>EARPKIGLVLSGGAARGLAHIGVLKALDEQG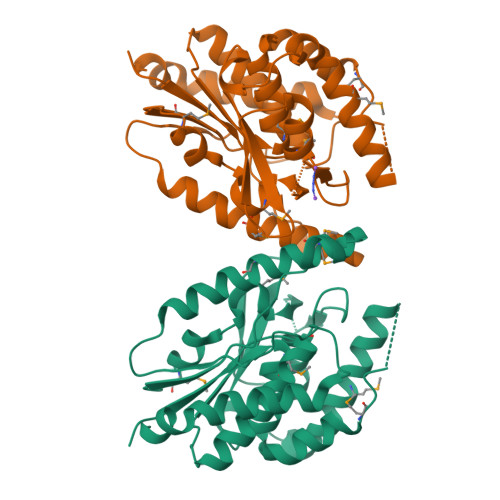IQIDAIAGTSMGAVVGGLYASGYTPAELERIALEMDWQQALSDAPPRKDVPFRRKQDDRDFLVKQKISFRDDGTLGLPLGVIQGQNLAMVLESLLVHTSDNRDFDKLAIPFRAVSTDIATGEKVVFRKGHLPQAIRASMSIPAVFAPVEIDGRLLVDGGMVDNIPVDVARDMGVDVVIVVDIGNPLRDRKDLSTVLDVMNQSITLMTRKNSEAQLATLKPGDVLIQPPLSGYGTTDFGRVPQLIDAGYRATTVLAARLAELRKPKDLNSEALDVARTPNQRKP[2x]> FLIKPYEGESLSHFLGRFRRANHLSASGLGTLAGIGAIVARWERFHFNPRPSQQELEAIASVVEVDAQRLAQMLPPAGVGMQHEPIRLCGACYAESPCHRIEWQYKSVWKCDRHQLKILAKCPNCQAPFKMPALWEDGCC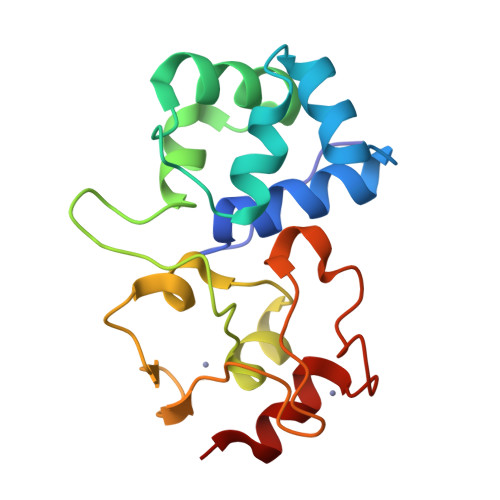HRCRMPFAEMAKLQK> GKAVIAIHGGAGAISRAQMSLQQELRYIEALSAIVETGQKMLEAGESALDVVTEAVRLLEECPLFNAGIGAV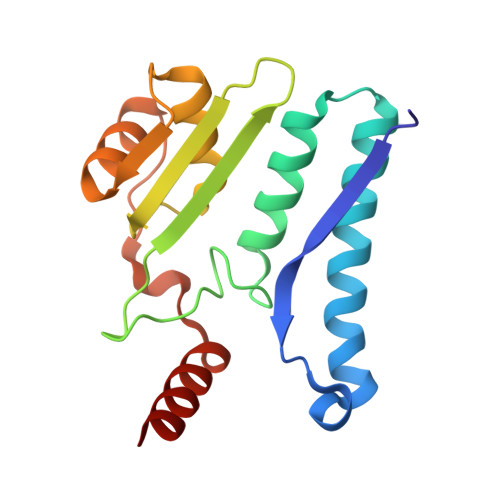FTRDETHELDACVMDGNTLKAGAVAGVSHLRNPVLAARLVMEQSPHVMMIGEGAENFAFARGMERVSPEIFSTSLRYEQLLAARKEGA>[2x]MSVDPMTYEAQFFGFTPQTCMLRIYIAFQDYLFEVMQAVEQVILKKLDGIPDCDISPVQIRKCTEKFLCFMKGHFDNLFSKMEQLFLQLILRIPSNILLPEDKCKETPYSEEDFQHLQKEIEQLQEKYKTELCTKQALLAELEEQKIVQAKLKQTLTFFDELHNVGRDHGTSDFRESLVSLVQNSRKLQNIRDNVEKESKRLKIS;>[2x]MTISRVKLLDTMVDTFLQKLVAAGSYQRFTDCYKCFYQLQPAMTQQIYDKFIAQLQTSIREEISDIKEEGNLEAVLNALDKIVEEGKVRKEPAWRPSGIPEKDLHSVMAPYFLQQRDTLRRHVQKQEAENQQLADAVLAGRRQVEELQLQVQAQQQAWQALHREQRELVAVLREPE;>[2x]MGTLQKCFEDSNGKASDFSLEASVAEMKEYITKFSLERQTWDQLLLHYQQEAKEILSRGSTEAKITEVKVEPMTYLGSSQNEVLNTKPDYQKILQNQSKVFDCMELVMDELQGSVKQLQAFMDESTQCFQKVSVQLGKRSMQQLDPSPARKLLKLQLQNPPAIHGSGSGSCQHHHHHH;>MGQAWQEASDNCFMDSDIKVLEDQFDEIIVDIATKRKQYPRKILECVIKTIKAKQEILKQYHPVVHPLDLKYDPDPAPHMENLKCRGETVAKEISEAMKSLPALIEQGEGFSQVLR[2x];>GPLGSMAASGLDHLKNGYRRRFCRPSRARDINTEQGQNVLEILQDCFEEKSLANDFSTNSTKSVPNSTRKIKDTCI[2x]

Kinetochores, multisubunit protein assemblies, connect chromosomes to spindle microtubules to promote chromosome segregation. The 10-subunit KMN assembly (comprising KNL1, MIS12, and NDC80 complexes, designated KNL1C, MIS12C, and NDC80C) binds microtubules and regulates mitotic checkpoint function through NDC80C and KNL1C, respectively. The 10-subunit KMN assembly consists of three complexes, the 4-subunit MIS12 complex (MIS12C), the 2-subunit KNL1 complex (KNL1C), and the 4-subunit NDC80 complex (NDC80C) (Bharadwaj et al., 2004, Cheeseman et al., 2004, De Wulf et al., 2003, Desai et al., 2003, Kline et al., 2006, McCleland et al., 2003, Nekrasov et al., 2003, Obuse et al., 2004, Pinsky et al., 2003, Westermann et al., 2003, Wigge and Kilmartin, 2001). Human MIS12C (also known as MIND complex or Mtw1 complex in Saccharomyces cerevisiae) contains the MIS12, PMF1, NSL1, and DSN1 subunits (synonyms are reported in Table S1A). Finally, MIS12C is a binding hub that connects the other two KMN complexes to CCAN through an interaction with CENP-C (Gascoigne et al., 2011, Hori et al., 2013, Hornung et al., 2011, Hornung et al., 2014, Liu et al., 2016, Maskell et al., 2010, Petrovic et al., 2010, Przewloka et al., 2011, Screpanti et al., 2011).

We speculated that the detachment of Head2 from the core of the MIS12C might, at least in part, explain our difficulties in obtaining well-ordered crystals of MIS12C. We therefore generated a deletion construct, referred to as MIS12CΔHead2 (i.e., lacking Head2). MIS12CΔHead2 retained CENP-C binding (see below) and readily crystallized with it in the absence of proteases. We determined the structure at 3.25 Å resolution as described in the STAR Methods. The Head1 and Stalk of MIS12CΔHead2 retain the overall organization and relative orientation observed in the crystal of complete MIS12C, except for a small rigid body movement of Head1 relatively to the stalk. In both complexes in the asymmetric unit of the MIS12CΔHead2:CENP-C1-71 crystals, clear electron density is only visible for residues 6–18 of CENP-C, whereas no density for the helical C-terminal segment is visible, probably due to crystal contacts involving MIS12C. A MIS12C construct lacking Head1 (MIS12CΔHead1) did not interact with CENP-C, while MIS12CΔHead2 bound CENP-C like MIS12CWT (even with higher affinity ). Indeed, the MIS12CΔHead2 construct, which also lacks Ser100DSN1 and Ser109DSN1, binds CENP-C in SEC experiments. Indeed, MIS12CΔHead2 bound FAMCENP-C1-21 in fluorescence polarization experiments with a Kd of 2.2 nM, i.e., almost 60-fold more tightly than MIS12CWT. We observed an equivalent increase in affinity with a shorter deletion mutant of MIS12C, which lacked only the 10-residue segment encompassing Ser100DSN1 and Ser109DSN1 (MIS12CDSN1Δ100–109). These results argue that segment 100–109 of DSN1 likely binds directly to the CENP-C binding site of MIS12C through an inter-subunit interaction, as depicted schematically in Figure 5C.> KAMHVAQPAVVLASSRGIASFVCEYASPGKATEVRVTVLRQADSQVTEVCAATYMMGNELTFLDDSICTGTSSGNQVNLTIQG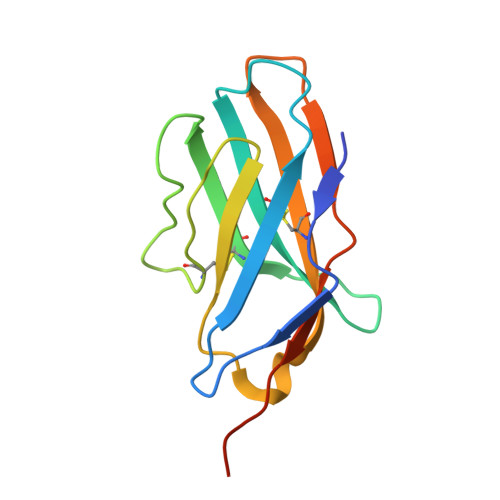LRAMDTGLYICKVELMYPPPYYLGIGNGAQIYVIDPEPCPDSD> GPKRIAX;> MGSSHHHHHHSSGLVPRGSTSEVIEDEKQFYSKAKTYWKQIPPTVDGMLGGYGHISSIDINSSRKFLQRFLREGPNKTGTSCALDCGAGIGRITKRLLLPLFREVDMVDITEDFLVQAKTYLGEEGKRVRNYFCCGLQDFTPEPDSYDVIWIQWVIGHLTDQHLAEFLRRCKGSLRPN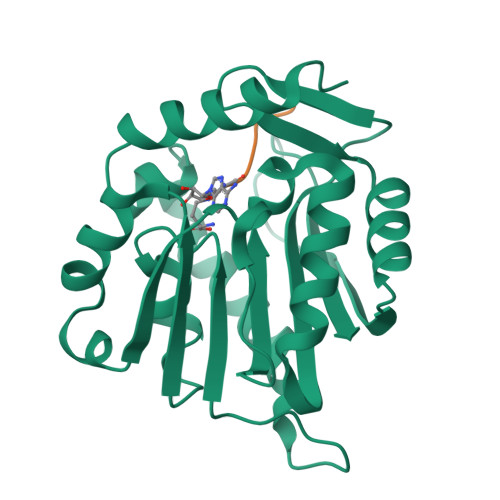GIIVIKDNMAQEGVILDDVDSSVCRDLDVVRRIICSAGLSLLAEERQENLPDEIYHVYSFALR> MHGGATTVNISTAEWWPKALNLDILSQHDRKTNPMGPDFNYQEEVKKLDVAALKQDLQALMTDSQDWWPADWGHYGGLMIRLTWHAAGTYRIADGRGGAGTGNQRFAPLNSWPDNTNLDKARRLLWPIKQKYGNKLSWADLIAYAGTIAYESMGLKTFGFAFGREDIWHPEKDIYWGPEKEWVPPSTNPNSRYTGDRELENPLAAVTMGLIYVNPEGVDGNPDPLKTAHDVRVTFARMAMNDEETVALTAGGHTVGKCHGNGNAALLGPEPEGADVEDQGLGWINKTQSGIGRNAVTSGLEGAWTPHPTQWDNGYFRMLLNYDWELKKSPAGAWQWEPINPREEDLPVDVEDPSIRRNLVMTDADMAMKMDPEYRKISERFYQDPAYFADVFARAWFKLTHRDMGPKARYIGPDVPQEDLIWQDPIPAGNRNYDVQAVKDRIAASGLSISELVSTAWDSARTYRNSDKRGGANGARIRLAPQKDWEGNEPDRLAKVLAVLEGIAAATGASVADVIVLAGNVGVEQAARAAGVEIVLPFAPGRGDATAEQ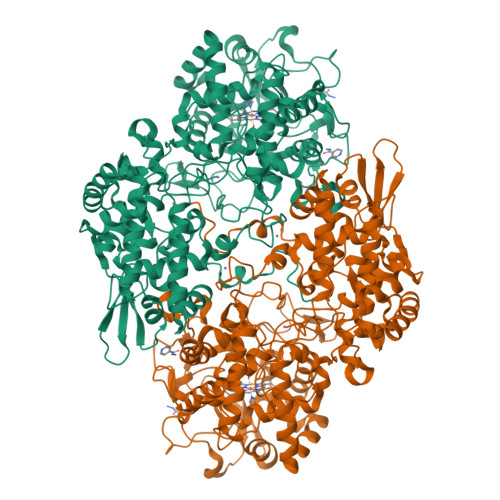TDTESFAVLEPIHDGYRNWLKQDYAATPEELLLDRTQLLGLTAPEMTVLIGGLRVLGTNHGGTKHGVFTDREGVLTNDFFVNLTDMNYLWKPAGKNLYEICDRKTNQVKWTATRVDLVFGSNSILRAYSELYAQDDNKEKFVRDFVAAWTKVMNADRFDLD> SATRANKDIFTLFDKKGQGAIAKDSLGDYLRAIGYNPTNQLVQDIINADSSLRDASSLTLDQITG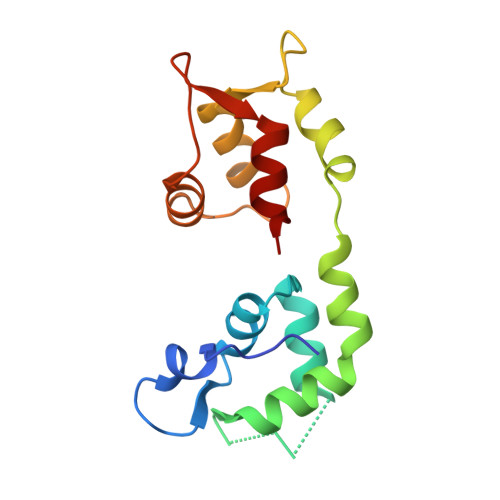LIEVNEKELDATTKAKTEDFVKAFQVFDKESTGKVSVGDLRYMLTGLGEKLTDAEVDELLKGVEVDSNGEIDYKKFIEDVLRQ3-[4-[2,3-dihydro-1H-inden-4-yl(methyl)amino]-6-(trifluoromethyl)pyrimidin-2-yl]oxypropanoic 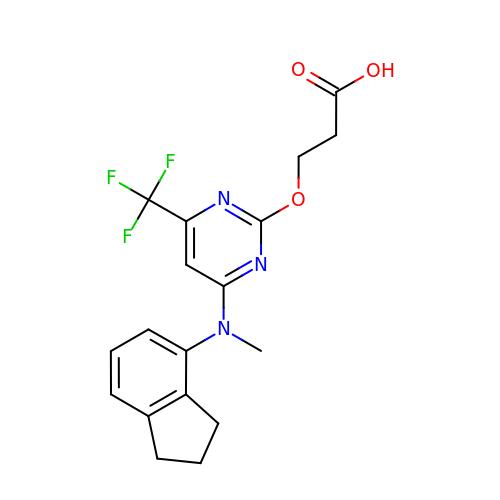acid | C18 H18 F3 N3 O3 | YMSJOQCCWIPKGF-UHFFFAOYSA-N>EQTNQIANKPQAIQWHTNLTNERFTTIAHRGASGYAPEHTFQAYDKSHNELKASYIEIDLQRTKDGHLVAMHDETVNRTTNGHGKVEDYTLDELKQLDAGSWFNKKYPKYARASYKNAKVPTLDEILERYGPNANYYIETKSPDVYPGMEEQLLASLKKHHLLNNNKLKNGHVMIQSFSDESLKKIHRQNKHVPLVKLVDKGELQQFNDQRLKEIRSYAIGLGPDYTDLTEQNTHHLKDLGFIVHPYTVNEKADMLRLNKYGVDGVFTNFADKY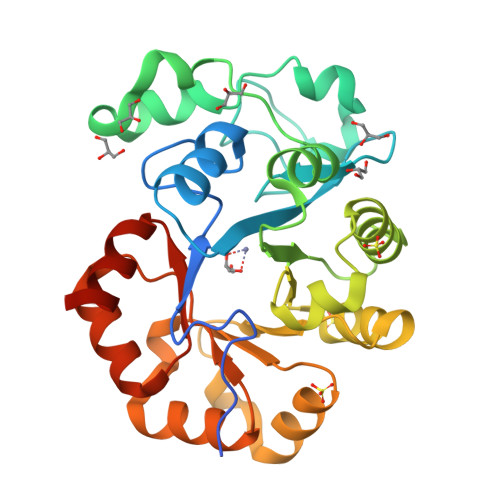KEVIKEGHHHHHH[6x]>GTGMESKYKEILLLTGLDNITDEELDRFKFFLSDEFNIATGKLHTANRIQVATLMIQNAGAVSAVMKTIRIFQKLNYMLLAKRLQEEKEKVDKQ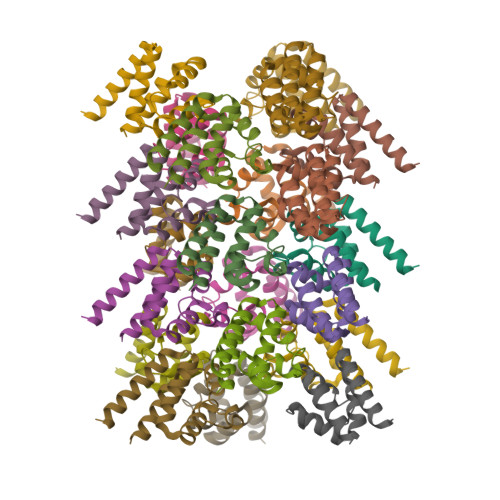YKSVTKPKPLSQAEMSPAASAAIRND[21x]>MQINLFLKQSTFSLLMALSLIACSEQKTETKSTPTEDSATTEHKVFPHKMPSEKPDMPLSAAAERMFSYPAPRVQDNELFSQFKYTRLKGFDYNNGDGTISRRDPSRPILVNGKYYIYYTKRDTKVPPIGWNRAKEATDEIPSTDWDLCEIWYATSEDGTTWKEEGVAIARPEKPKPGWRSVATPDILVWKGKYYLYYQAFNEPSGLRGDWCPVSVSYADSPDGPWTHGGDSVIPFGKKGEWDQDATHDPQPIVYKGKIHLYYKAAYNKWPDIRDKYAVGHGLAIADDPLGPFEKHPLNPVMTSGHETTYFPFKEGVATLAIKDGNERYTMQYAKDGVNFEIASVVSLAPTAAAPFAADAFTDSGNGRGV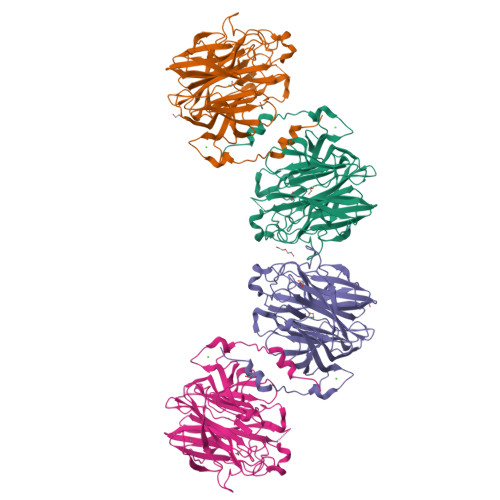TWGLCHFTNASNNPKKGYSIIARFDCDLSLDVDDPFYKNTGVWHRPEVYFAQAPRKNLSPEGR[4x]Bacterial infections including Salmonellosis and Shigellosis affect millions of people every year. These bacteria use a T3SS to secrete virulence factors to manipulate host cells. The T3SS is a multi-component system that forms a continuous protein transport channel through the two bacterial membranes and the periplasmatic space that extends into the surrounding medium by a needle structure. Tip proteins, which bind to the distal end of the T3SS needle, are thought to play an important role in this process. SipD from S. typhimurium, IpaD from Shigella flexneri and BipD from Burkholderia mallei are tip proteins that are thought to interact with their corresponding needle subunits PrgI, MxiH and BsaL, respectively, to make the needle tip complex.

Here, we address the questions of how the Salmonella SipD interacts with PrgI and deoxycholate and the mechanistic consequences of the assembly of the T3SS needle tip complex. We could show that two different proteins, structurally conserved in many pathogenic bacteria, bind each other to constitute the needle tip of the transport system. Multiple copies of both proteins constitute the tip of the transport system in what may represent the open state of the needle.

>[2x]GSHMATPWSGYLDDVSAKFDTGVDNLQTQVTEALDKLAAKPSDPALLAAYQSKLSEYNLYRNAQSNTVKVFKDIDAAIIQNFRGGSGGTTISDAEIWDMVSQNISAIGDSYLGVYENVVAVYTDFYQAFSDILSKMGGWLLPGKDGNTVKLDVTSLKNDLNSLVNKYNQINSNTVLFPAQSGSGVKVATEAEARQWLSELNLPNSCLKSYGSGYVVTVDLTPLQKMVQDIDGLGAPGKDSKLEMDNAKYQAWQSGFKAQEENMKTTLQTLTQKYSNANSLYDNLVKVLSSTISSSLETAKSFLQG>[2x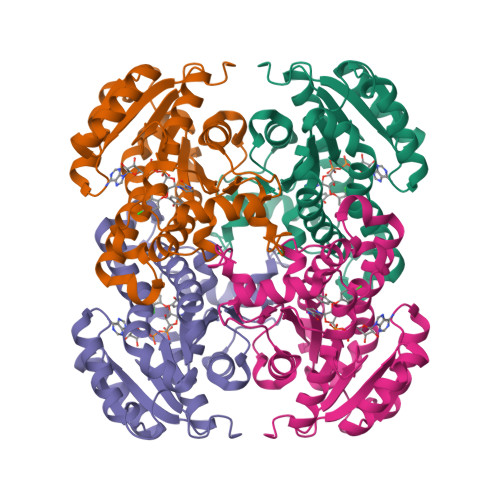]HHHHHHENLYFQSMLLKGQRFVVTGIASKLSIAWAIAESLHREGAQLILTYPNDKIKKRVDMAAEAFDAVAVIECDVGSDESIQVCFDEIAKHWGVGDDKGIDGIVHAIGFAPADQLDGDFTQATTREGSQIAHDISSYSFVALAKAGRELLAARQGSLLTLTYEGSISVLPNYNVMGMAKASLEASVRYLASSLGGEGIRVNAISAGPIRTLAASGIKSFRRMLDVSEKIAPLQRNVSQEEVGNAALFLLSPWASGITGEILFVDAGFNTVAISEKIMMMAGDGEQ> GSHMTYVSLADLERAARDVLPGEIFDFLAGGSGTEASLVANRTALERVFVIPRMLRDLTDVTTEIDIFGRRAALPMAVAPVAYQRLFHPEGELAVARAARDAGVPYTICTLSSVSLEEIAAVGGRPWFQLFWLRDEKRSLDLVRRAEDAGCEAIVFTVDVPWMGRRLRDMRNGFALPEWVTAANF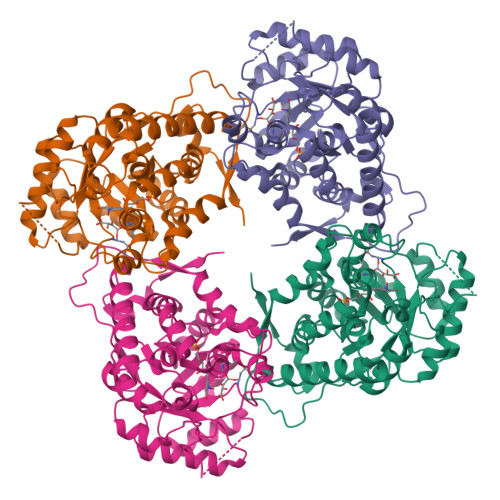DAGTAAHRRTQGVSAVADHTAREFAPATWESVEAVRAHTDLPVVLKGILAVEDARRAVDAGAGGIVVSNHGGRQLDGAVPGIEMLGEIVAAVSGGCEVLVDGGIRSGGDVLKATALGASAVLVGRPVMWALAAAGQDGVRQLLELLAEEVRDAMGLAGCESVGAARRLNTKLGVV> GPLGSQPAERGRNPQVRLLSAEQSMSKVQFRMDNLQFTGVQTSKGVAQVPTFTEGVNISEKGTPILPILSRSLAVSETRAMKVEVVSSKFI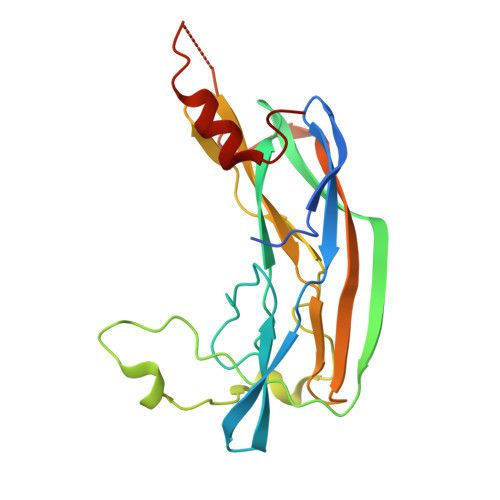EKKDVLIAPSKGVISRAENPDQIPYVYGQSYNEDKFFPGEIATLSDPFILRDVRGQVVNFAPLQYNPVTKTLRIYTEIVVAVSETAEAGQNTISLVKNSTFTGFEDIYKSVFMNYEATR> CGGPFELWEPNTTFSSTNFPNSYPNLAFCVWILNAQKGKNIQLHFQEFDLENINDVVEIRDGEEADSLLLAVYTGPGPVKDVFSTTNRMTVLLITNDVLARGGFKANFTTGYHLGIPEPCKADHFQCKNGECVPLVNLCDGHLHCEDGSDEADCVRFFNGTTNNNGLVRFRIQSIWHTACAENWTTQISNDVCQLLGLGSGNSSKPIFPTDGGPFVKLNTAPDGHLILTPSQQCLQDSLIRLQCNHKSCGKKLAAQDITPK;> IVGGSNAKEGAWPWVVGLYYGGRLLCGASLVSSDWLVSAAHCVYGRNLEPSKWTAILGLHMKSNLTSPQTVPRLIDEIVINPHYNRRRKDNDIAMMHLEFKVNYTDYIQPICLPEENQVFPPGRNCSIAGWGTVVYQGTTANILQEADVPLLSNERCQQQMPEYNITENMICAGYEEGGIDSCQGDSGGPLMCQENNRWFLAGVTSFGYKCALPNRPGVYARVSRFTEWIQSFLH

Human enteropeptidase (hEP), also known as enterokinase, is an essential enzyme in food digestion and is localized at the brush border of the duodenal and jejunal mucosa. Activated hEP can stimulate the conversion of trypsinogen to trypsin via cleavage of a specific trypsinogen activation peptide, namely Asp-Asp-Asp-Asp-Lys (DDDDK), which is highly conserved in vertebrates. However, the mechanism of hEP activation remains to be established. hEP contains a multi-domain heavy chain and a catalytic light chain, linked by a disulfide bond. The functions of these domains and motifs may be involved in protein anchoring, macromolecular substrate recognition and inhibitor specificity. The light chain is homologous to trypsin-like serine proteinases with a typical Asp-His-Ser (D-H-S) catalytic triad responsible for peptidase activity.

Upon cleavage of the hEP into heavy and light chains by trypsin, the enzyme became fully active as shown by the protease activity assay. The protruding LCM region was not resolved in the active hEP structure even after extensive 3D classifications. There was also no evidence of cleavage of the LCM domain as we observed only two bands, corresponding to the intact heavy and light chains, upon activation. This set of results indicated increasing dynamics of LCM relative to the hEP-core upon activation. Inspection of the cryo-EM structure of this active hEP-core at 3.2 Å resolution revealed an overall shape equivalent to that of the inactive state. Superposition of the hEP-core regions of the active and inactive states revealed additional density near the catalytic site in the active state, corresponding to the surface loops L1, L2 and LD not resolved in the inactive state. The IVGG sequence was observed to be flipped by ~180 degrees, with Ile785 shifted by ~16.6 Å. The newly exposed N-terminal amino group of Ile785 formed a salt bridge with the side chain of Asp970 to stabilize loop L1. Upon activation, the conformation of the catalytic triad Asp876-His825-Ser971 appeared to have remained unchanged. Upon activation of the zymogen, the flexible L1, L2 and LD loops form a complete and rigid catalytic pocket ready for performing catalysis.> MFARLIRYFQEARAELARVTWPTREQVVEGTQAILLFTLAFM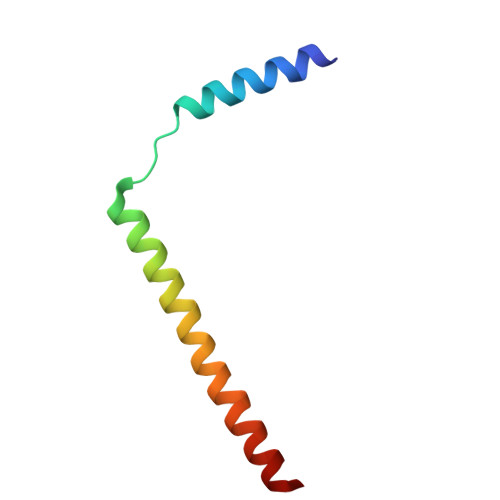VILGLYDTVFRFLIGLLR>LPEGAALTEKTDIFESGRNGKPNKDGIKSYRIPALLKTDKGTLIAGADERRLHSSDWGDIGMVIRRSEDNGKTWGDRVTITNLRDNPKASDPSIGSPVNIDMVLVQDPETKRIFSIYDMFPEGKGIFGMSSQKEEAYKKIDGKTYQILYREGEKGAYTIRENGTVYTPDGKATDYRVVVDPVKPAYSDKGDLYKGNQLLGNIYFTTNKTSPFRIAKDSYLWMSYSDDDGKTWSAPQDITPMVKADWMKFLGVGPGTGIVLRNGPHKGRILIPVYTTNNVSHLNGSQSSRIIYSDDHGKTWHAGEAVNDNRQVDGQKIHSSTMNNRRAQNTESTVVQLNNGDVKLFMRGLTGDLQVATSKDGGVTWEKDIKRYPQVKDVYVQMSAIHTMHEGKEYIILSNAGGPKRENGMVHLARVEENGELTWLKHNPIQKGEFAY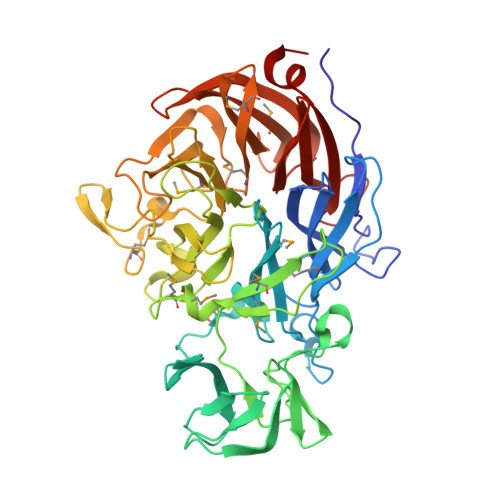NSLQELGNGEYGILYEHTEKGQNAYTLSFRKFNWDFLSKDL[2x]>[6x]G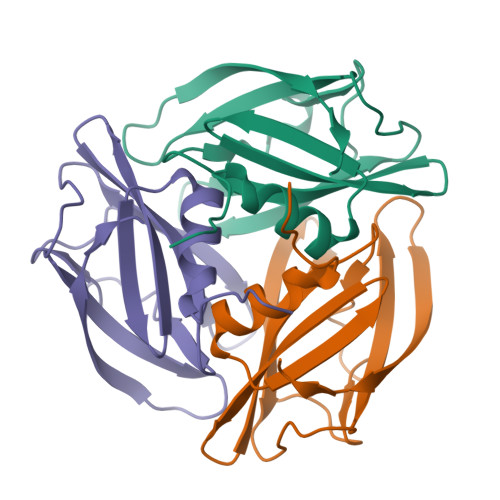AQAGSGISVANTGVAVQAGNGISVTSTGVAVKAGNGIQVNTNGVGLKSTAWINVMCGLHNATFYVYSSYFCAFFCNYSNGCVAYVYGRGAFYLSTVSGDIKLNSVSPNQILAMTGGSSSAVTMMSWTSTKAAEGISLEYQRKSLINSSSISGSASLVSAP> VEATAQETDRPRFSFSIAAREGKARTGTIEMKRGVIRTPAFMPVGTAATVKALKPETVRATGADIILGNTYHLMLRPGAERIAKLGGLHSFMGWDRPILTDSGGYQVMSLSSLTKQSEEGVTFKSHLDGSRHMLSPERSIEIQHLLGSDIVMAFDECTPYPATPSRAASSMERSMRWAKRSRDAFDSRKEQAENAALFGIQQGSVFENLRQQSADALAEIGFDGYAVGGLAVGEGQDEMFRVLDFSVPMLPDDKPHYLMGVGKPDDIVGAVERGIDMFECVL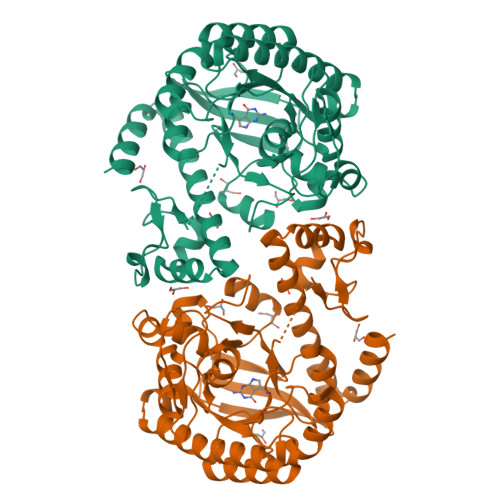PTRSGRNGQAFTWDGPINIRNARFSEDLKPLDSECHCAVCQKWSRAYIHHLIRAGEILGAMLMTEHNIAFYQQLMQKIRDSISEGRFSQFAQDFRARYFA> SSGMQIGKIIKVSGPLVMAENMSEASIQDMCLVGDLGVIGEIIEMRQDVASIQVYEETSGIGPGEPVRSTGEALSVELGPGIISQMFDGIQRPLDTFMEVTQSNFLGRGVQLPALDHEKQWWFEATIEEGTEVSAGDIIGYVDETKIIQHKIMVPNGIKGTVQKIESGSFTIDDPICVIETEQGLKELTMMQKWPVRRGRPIKQKLNPDVPMITGQRVIDTFFPVTKGGAAAVPGPFGAGKTVVQHQIAKWSDVDLVVYVGCGERGNEMTDVVNEFPELIDPNTGESLMERTVLIANTSNMPVAAREASIYTGITIAEYFRDMGYDVAIMADSTSRWAEALREMSGRLEEMPGDEGYPAYLGSRLAEYYERSGRVIALGSDQREGSITAISAVSPSGGDISEPVTQNTLRVVKVFWGLDSSLAQKRHFPSINWIQSYSLYSTEVGRYMDQILQQDWSDMVTEGMRILQEEEQLNEIVRLVGIDSLSDNDRLTLEVAKSIREDYLQQNAFDDVDTFTSREKQFNMLKVILTFGKEARKALSLGAYFNE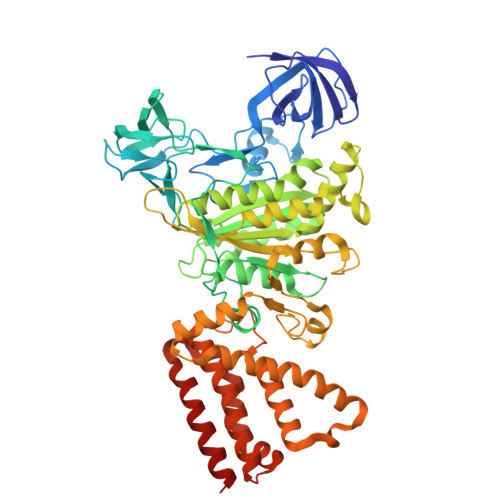IMEGTVAVRERISRSKYIPEEELAKISSINEEIKETIQLIVSEGGMTDD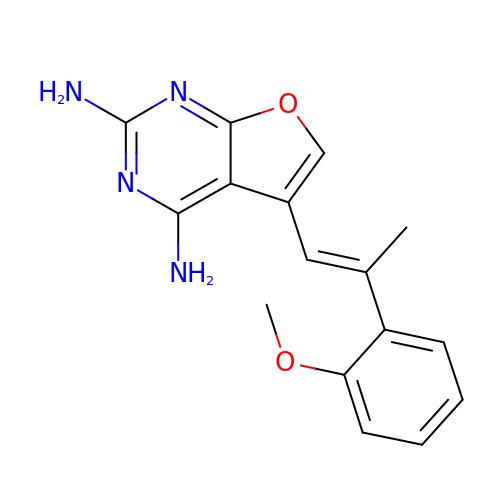5-[(1E)-2-(2-methoxyphenyl)prop-1-en-1-yl]furo[2,3-d]pyrimidine-2,4-diamine | C16 H16 N4 O2 | JXICVPBZQSPDOK-VQHVLOKHSA-N>[4x]CGC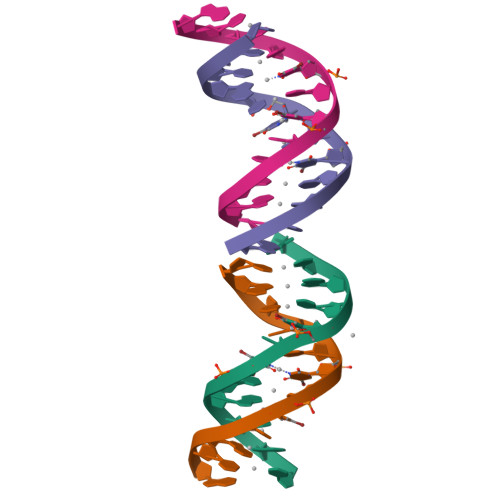GCUCUCGCG6-(6-AMINO-PURIN-9-YL)-2-THIOXO-TETRAHYDRO-2-FURO[3,2-D][1,3,2]DIOXAPHOSPHININE-2,7-DIOL | C10 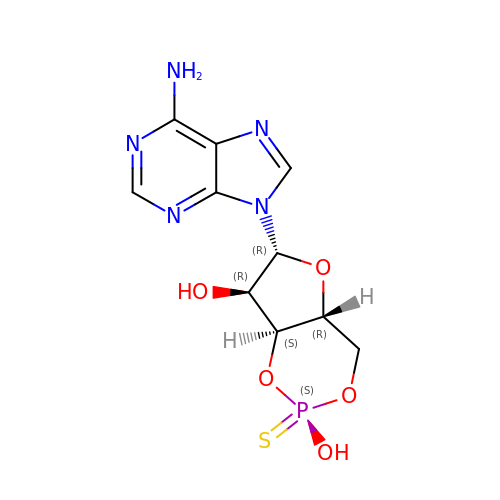H12 N5 O5 P S | SMPNJFHAPJOHPP-LHKKBNDGSA-N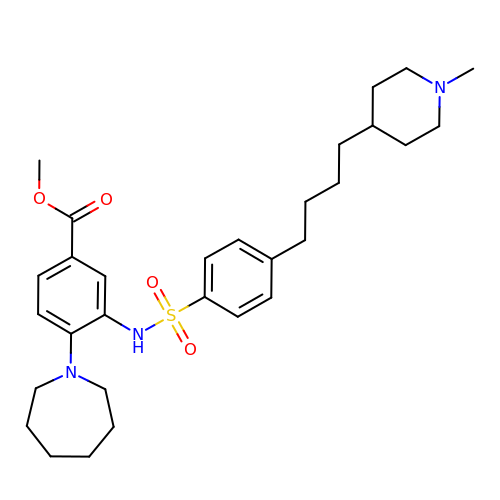methyl 4-(azepan-1-yl)-3-[[4-[4-(1-methylpiperidin-4-yl)butyl]phenyl]sulfonylamino]benzoate | C30 H43 N3 O4 S | HLBWOHTYZSIRPE-UHFFFAOYSA-N> ILKEPV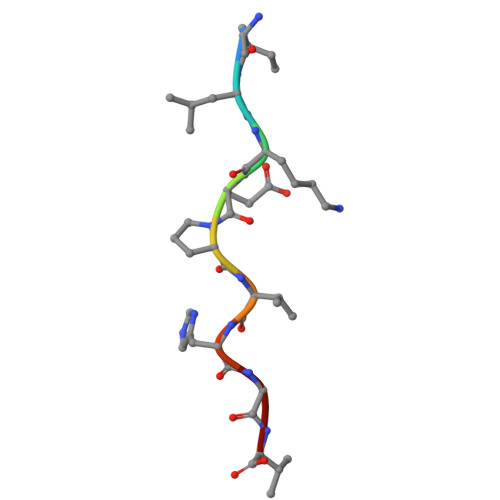HGV> TICADGTSVANGACCKLIPVVKDLTENLFEGECGDAAHGALRLVFHDAIAISPTLGGGGADGSIAVFNATELTFHANTGIDDVLDAVGPFLLKHSDVMTPGDFIQLAGAVSLTQCNGAPRVKFVMGRPPPKAAAPNLLVPEPFDSVATILQRFGELGFTKEETVAVIGGSHSVAGADDIVPNEQGIPFDQTPSIFDTQIFVDVQLRGTMIPGNGTTEGEVETAVPGTVRLQSDHLLARDASTSCIWQSFVNQQSKMAQVFGEAIFKMSLLGQTQSKLIDCSEVIPRAIPFSHGPATLPPGQTLKDIEQACAASPFPTLSTQPGPVTSVPAIPQAD

Manganese peroxidases (MnPs) are, together with lignin peroxidases and versatile peroxidases, key elements of the enzymatic machineries secreted by white-rot fungi to degrade lignin, thus providing access to cellulose and hemicellulose in plant cell walls. The primary mechanism involves the MnP oxidation of Mn2+ to Mn3+ and the subsequent formation of chelates with fungal dicarboxylic acids. The molecular structures of Ape-MnP1 and Cst-MnP1, which share 50% amino acid sequence identity, are characteristic of ligninolytic peroxidases.

The refined structures of the two MnPs with manganese yielded near complete models. Thus, the model of Ape-MnP1 consists of 335 amino acids (from Thr1 of the mature protein to Asp335) and that of Cst-MnP1 includes 331 residues (from Val1 of the mature protein to Ser331). Besides the amino acids of the polypeptide sequences, final models, crystallized in the presence of manganese, contain a heme prosthetic group, two structural calcium ions, and a substrate Mn2+ ion, as well as 180 (Ape-MnP1) and 171 (Cst-MnP1) solvent molecules (with three Mg2+ ions from the crystallization medium also present in the Cst-MnP1 structure). Mn2+ binding was confirmed by anomalous difference electron density maps. As a consequence, using Ape-MnP1 and Cst-MnP1 as representatives of the subfamilies they belong to, we renamed both subfamilies as MnP-DDQ, with a manganese oxidation site made up of Asp/Asp/Gln; and MnP-ED, with a manganese oxidation site formed by Glu/Asp. It was surprising to find that the MnP-DDQ subfamily differs from previously characterized MnPs in two of the three residues involved in Mn2+ coordination, with Asp35 and Gln333 in Ape-MnP1 occupying the position of two glutamate residues in short and long/extra-long MnPs. Moreover, this is the first MnP subfamily described that includes a residue of the C-terminal end contributing to the Mn2+ oxidation site. The different orientation of the Asp35 side chain in the structures of substrate-bound and substrate-free Ape-MnP1, and the absence of Gln333 in the crystal structure of the Mn-free enzyme, confirm the mobility of these residues, a behavior that has also been demonstrated for the two glutamates of the Mn2+ oxidation site in previously characterized MnPs. Once coordinated, Gln333 also contributes to anchoring the C-terminal end of the enzyme, where this amino acid is located, restraining the mobility of this region of the protein. The kinetic constants of Ape-MnP1-Q333P confirmed that Gln333 participates in Mn2+ binding (a 172-fold decrease in Mn2+ affinity was observed for the mutated variant) but not in its oxidation (kcat was hardly impaired).> GSMVEATAQETDRPRFSFSIAAREGKARTGTIEMKRGVIRTPAFMPVGTAATVKALKPETVRATGADIILGNTYHLMLRPGAERIAKLGGLHSFMGWDRPILTDSGGYQVMSLSSLTKQSEEGVTFKSHLDGSRHMLSPERSIEIQHLLGSDIVMAFDECTPYPATPSRAASSMERSMRWAKRSRDAFDSRKEQAENAALFGIQQGSVFENLRQQSADALAEIGFDGYAVGGLAVGEGQDEMFRVLDFSVPMLPDDKPHYLMGDGKPDDIVGAVERGIDMFDCVLPTRSGRNGQAFTWDGPINIRNARFSEDLKPLDSECHCAVCQKWSRAYIHHLIRAGEILGAMLMTEHNIAFYQQLMQKIRDSI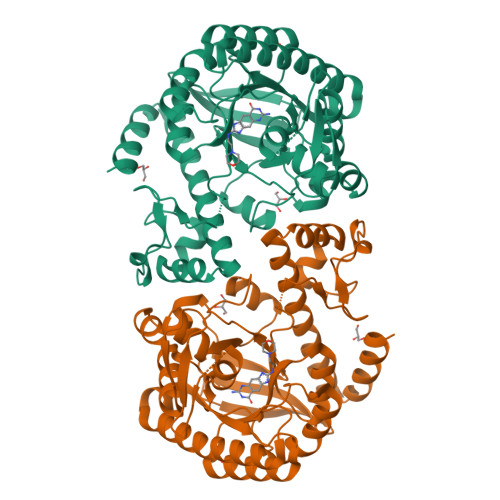SEGRFSQFAQDFRARYFARNS>MGSSHHHHHHSSGLVPRGSHMSTAGDDAVGVPPACGGRSDAVGVPQLARESGAMRDQDCSGELLRSPTHNGHLLVGALKRHQNKPVLFLGDTRLTGGQLADRISQYIQAFEALGAGTGVAVGLLSLNRPEVLMIIGAGQARGYRRTALHPLGSLADHAYVLNDAGISSLIIDPNPMFVERA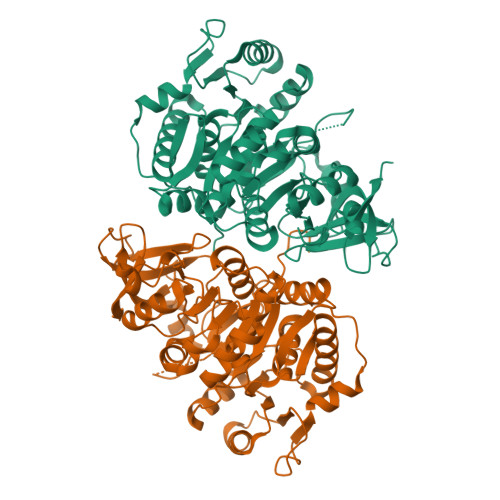LALLEQVDSLQQILTIGPVPDALKHVAVDLSAEAAKYQPQPLVAADLPPDQVIGLTYTGGTTGKPKGVIGTAQSIATMTSIQLAEWEWPANPRFLMCTPLSHAGAAFFTPTVIKGGEMIVLAKFDPAEVLRIIEEQRITATMLVPSMLYALLDHPDSHTRDLSSLETVYYGASAINPVRLAEAIRRFGPIFAQYYGQSEAPMVITYLAKGDHDEKRLTSCGRPTLFARVALLDEHGKPVKQGEVGEICVSGPLLAGGYWNLPDETSRTFKDGWLHTGDLAREDSDGFYYIVDRVKDMIVTGGFNVFPREVEDVVAEHPAVAQVCVVGAPDEKWGEAVTAVVVLRSNAARDEPAIEAMTAEIQAAVKQRKGSVQAPKRVVVVDSLPLTGLGKPDKKAVRARFWEGAGRAVG[2x]> STQNLGNSLMRVFSKEAT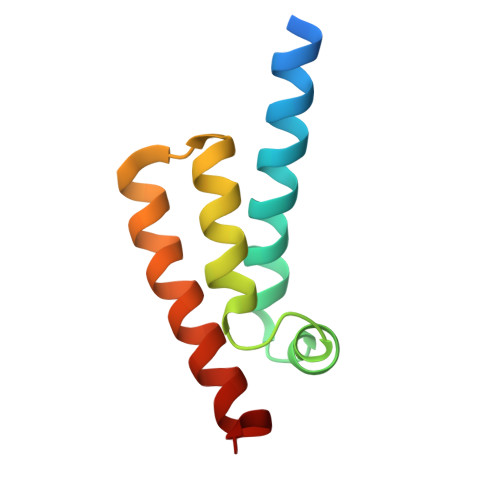RKYYLDLFKRADFTANLPKLAKKGGPDRLNDALKKLRKAGISEEKFAELKGAAAKYADDWYRIYGK>ANPCCSNPCQNRGECMSTGFDQYKCDCTRTGFYGENCTTPEFLTRIKLLLKPTPNTVHYILTHFKGVWNIVNNIPFLRSLIMKYVLTSRSYLIDSPPTYNVHYGYKSWEAFSNLSYYTRALPPVADDCPTPMGVKGNKELPDSKEVLEKVLLRREFIPDPQGSNMMFAFFAQHFTHQFFKTDHKRGPGFTRGLGHGVDLNHIYGETLDRQHKLRLFKDGKLKYQVIGGEVYPPTVKDTQVEMIYPPHIPENLQFAVGQEVFGLVPGLMMYATIWLREHNRVCDILKQEHPEWGDEQLFQTSRLILIGETIKIVIEDYVQHLSGYHFKLKFDPELLFNQQFQYQNRIASEFNTLYHWHPLLPDTFNIEDQEYSFKQFLYNNSILLEHGLTQFVESFTRQIAGRVAGGRNVPIAVQAVAKASIDQSREMKYQSLNEYRKRFSLKPYTSFEELTGEKEMAAELKALYSDIDVMELYPALLVEKPRPDAIFGETMVELGAPFSLKGLMGNPICSPQYWKPSTFGGEVGFKIINTASIQSLICNNV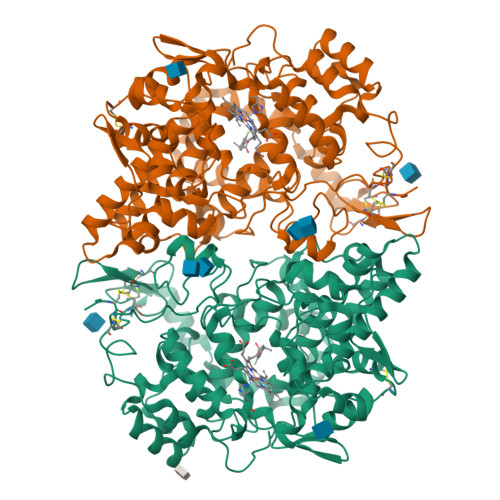KGCPFTSFNVQDPQPTKTA[4x]> IVGGYTCGANTVPYQVSLNSGYHFCGGSLLNSQWVVSAAHCYKSGIQVRLGEDNINVVEGNEQFISASKSIVHPSYNSETYNNDIMLIKLKSAASLNSRVA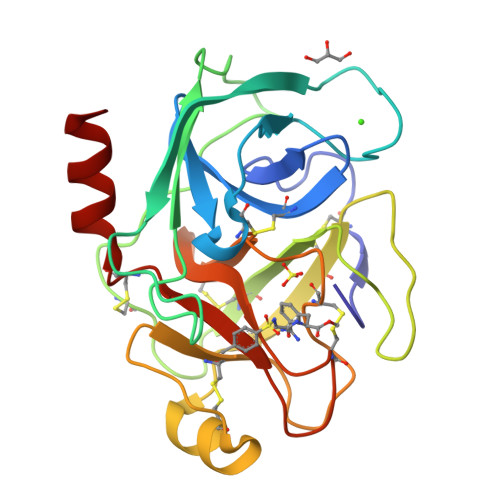SISLPTSCASAGTQCLISGWGNTKSSGTSYPDVLKCLKAPILSDSSCKSASSFIITSNMFCAGYLEGGKDACQGDSGGPVVCSGKLQGIVSWGSGCAQKNKPGIYTKVCNYVSWIKQTIASN> 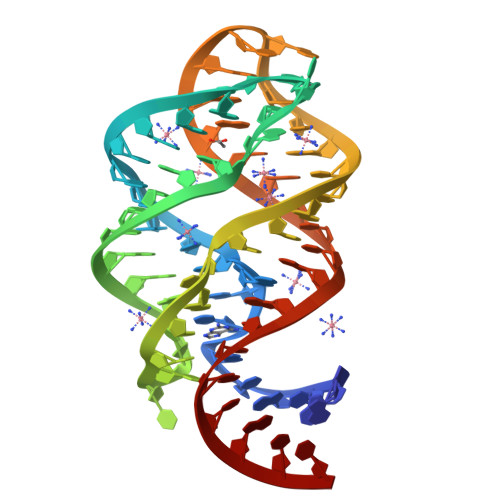GACAUAUAAUCGCGUGGAUAUGGCACGCAAGUUUCUACCGGGCACCGUAAAUGUCCGAUUAUGUC> AFTLADRVTEEMLADKAALVVEVVEENYHDAPIVGIAVVNEHGRFFLRPETALADPQFVAWLGDETKKKSMFDSKRAAVALKWKGIELCGVSFDLLLAAYLLDPAQGVDDVAAAAKMKQYEAVRPDEAVYGKGAKRAVPDEPVLAEHLVRKAAAIWALERPFLDELRRNEQDRLLVELEQPLSSILAEMEFAGVKVDTKRLEQMGEELAEQLRTVEQRIYELAGQEFNINSPKQLGVILFEKLQLPVLKKTKTGYSTSADVLEKLAPYHEIVENILHYRQLGKLQSTYIEGLLKVVRPDTKKVHTIFNQALTQTGRLSSTEPNLQNIPIRLEEGRKIRQAFVPSESDWLIFAADYSQIELRVLAHIAEDDNLMEAFRRDLDIHTKTAMDIFQVSEDEVTPNMRRQAKAVNFGIVYGISDYGLAQNLNISRKEAAEFIERYFESFPGVKRYMENIVQEAKQKGYVTTLLHRRRYLPDITSRNFNVRSFAERMAMNTPIQGSAADIIKKAMIDLNARLKEERLQARLLLQVHDELILEAPKEEMERLCRLVPEVMEQAVTLRVPLKVDYHYGSTWYDAK

In a surprising twist to this paradigm, a naturally occurring bacterial DNA polymerase I member isolated from Geobacillus stearothermophilus (Bst) exhibits an innate ability to reverse transcribe RNA and other synthetic congeners (XNAs) into DNA. Here, we describe two X-ray crystal structures of Bst DNA polymerase that capture the post-translocated product of DNA synthesis on templates composed entirely of FANA and TNA. The structures reveal a Y-shaped architecture common to A-family polymerases that encompasses the catalytic and exonuclease domains of the enzyme. The catalytic domain is further divided into the finger, palm, and thumb subdomains with the P/T duplex bound in a groove defined by the palm and thumb subdomains.

The only exception was the FANA template, which contained uridine residues in place of thymidine residues, as FANA thymidine amidites are not commercially available. The crystal structures were solved to resolutions of 1.6 and 1.9 Å for the FANA and TNA bound structures, respectively. However, the post-translocated product observed in the FANA structure reveals formation of the n + 2 nucleotide addition product indicating that the polymerase underwent two rounds of catalysis. The first nucleotide addition generated the correct fA6-dT10 Watson–Crick base pair, while the subsequent addition produced an fU5-dT11 mispair at the n + 2 position. Relative to a previously solved Bst DNA polymerase structure for the natural n + 2 translocated product, the misincorporated dT11 nucleotide occupies the same position but exhibits greater rise, tilt, and twist than the correct dT5–dA11 Watson–Crick pair observed in the natural system. The second nucleotide adduct, which is presumably due to prolonged incubation of the enzyme with the TTP substrate, provides structural evidence for a fU–dT mispair, which could be relevant to future studies that examine the fidelity of DNA synthesis on XNA templates. By contrast, FANA maintains the same C1′-exo conformation observed in the solution structure of a FANA duplex. The shorter P···P distance of the TNA strand is due to the backbone repeat unit of TNA, which has 5 atoms (or bonds) rather than the normal 6-atom backbone repeat unit found in DNA and RNA. Both strands of the DNA/FANA duplex have P···P distances of ∼6.6 Å, which closely approximates the all-natural DNA system. By comparison, the DNA/FANA duplex is nearly identical to a standard DNA/DNA with a normal six-atom backbone repeat unit. Several unique interactions are observed between active site residues, mostly from the palm subdomain, and the chimeric duplexes that are not observed in the natural system, including eight new interactions to the DNA/FANA duplex and 13 new interactions to the DNA/TNA duplex.> MEVVMDNIIDVSIPVAEVVDKHPEVLEILVELGFKPLA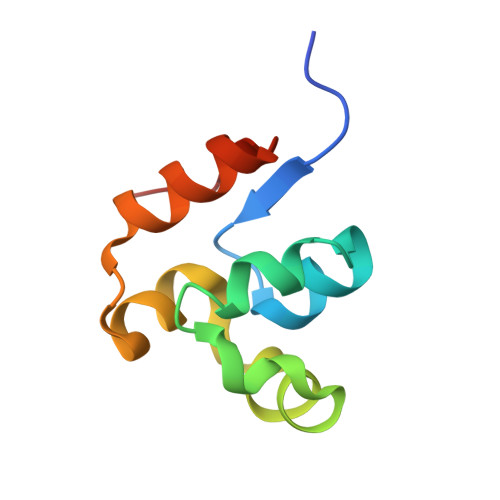NPLMRNTVGRKVSLKQGSKLAGTPMDKIVRTLEANGYEVIGLD>MKKSLLGLTFASLMFSAGSAVAADYKIDKEGQHAFVNFRIQHLGYSWLYGTFKDFDGTFTFDEKNPAADKVNVTINTTSVDTNHAERDKHLRSADFLNTAKYPQATFTSTSVKKDGDELDITGDLTLNGVTKPVTLE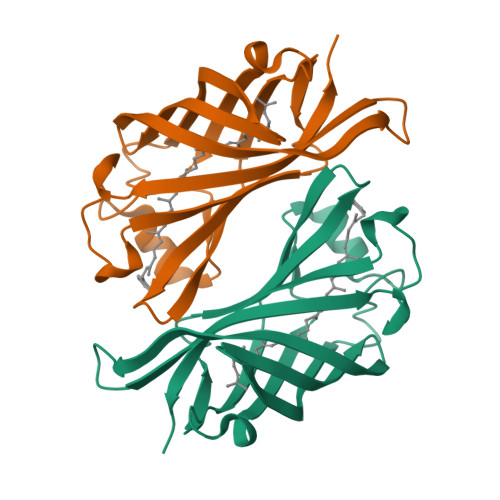AKLIGQGDDPWGGKRAGFEAEGKIKLKDFNIKTDLGPASQEVDLIISVEGVQQK[4x]> MPVLNLNDPQAVERYEEFMRQSPYGQVTQDLGWAKVKNNWEPVDVYLEDDQGAIIAAMSMLLGDTPTDKKFAYASKGPVMDVTDVDLLDRLVDEAVKALDGRAYVLRFDPEVAYSDEFNTTLQDHGYVTRNRNVADAGMHATIQPRLNMVLDLTKFPDAKTTLDLYPSKTKSKIKRPFRDGVEVHSGNSATELDEFFKTYTTMAERHGITHRPIEYFQRMQAAFDADTMRIFVAEREGKLLSTGIALKYGRKIWYMYAGSMDGNTYYAPYAVQSEMIQW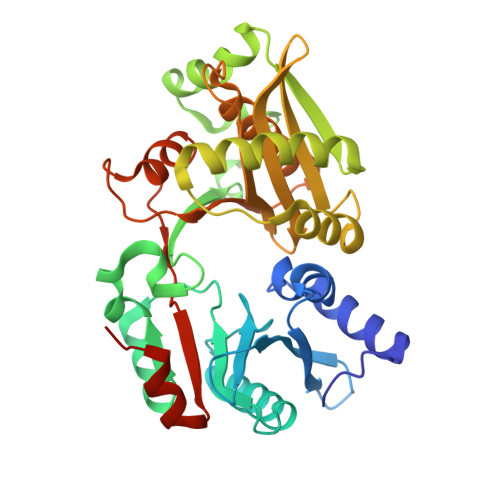ALDTNTDLYDLGGIESESTDDSLYVFKHVFVKDAPREYIGEIDKVLDPEVYAELVKDGHHHHHH Double-drugging via active and allosteric sites is a recently developed approach to overcome these obstacles. Herein, we provide the quantitative framework for double-drugging using two targets: Aurora A kinase (AurA) and Abl. Both kinases participate in various cellular pathways, and their dysregulation results in a multitude of cancers, such as breast cancer and leukemia. We find that both orthosteric and allosteric ligands exhibit preferred binding to the active or inactive states and that cooperativity occurs by shifting this active–inactive conformational equilibrium through long-range allosteric networks that are encoded for natural regulation of those kinases.

Intrigued by the synergistic effect of SKI and asciminib on Abl activity, we structurally characterized this ternary complex by cocrystallization, resulting in a 2.86 Å crystal structure of Abl64–510-SKI-asciminib [inactive, DFGin, BLBplus (29, 30)]. First, we note that the entire N-terminal lobe is ~30° twisted only for Abl64–510-SKI-asciminib, when aligned by the regulatory domains. Second, the α-C helix is adopting the “out” position resulting from this N-lobe twist, since an α-C helix “in position” would clash with strands β4 and β5. In consequence, the canonical salt bridge between K290 and E305, a hallmark of an active kinase, is broken in our structure, whereas D400 (DFG-motif) is positioned in the “in” position. We note, that the orthosteric site is fully occupied by SKI and the twisted N-lobe aids in forming this tightly packed binding pocket. In fact, K290 located on β3 strand is wrapping over SKI burying the inhibitor in Abl’s orthosteric site. Besides extensive van der Waals interactions between SKI and Abl, the quinazoline ring of SKI shares two hydrogen bonds with Abl, one between the side chain hydroxyl of T334 on β-strand 5 and N-2 of SKI as well as between the amide of M337 and N-0 of SKI. When compared to other closed Abl structures, we find an extended domain interface between SH3, linker, and N-lobe of the kinase domain, which explains the positive cooperativity between SKI and asciminib. Moreover, S248 (located on the linker) forms a hydrogen bond with D96 in the SH3 domain, which is only present in the ternary complex of Abl64–510-SKI-asciminib. We conclude that our complex of Abl64–510-SKI-asciminib represents the only example of a fully closed and inactive Abl structure.

>[2x]GNLFVALYDFVASGDNTLSITKGEKLRVLGYNHNGEWCEAQTKNGQGWVPSNYITPVNSLEKHSWYHGPVSRNAAEYLLSSGINGSFLVRESESSPGQRSISLRYEGRVYHYRINTASDGKLYVSSESRFNTLAELVHHHSTVADGLITTLHYPAPKRNKPTVYGVSPNYDKWEMERTDITMKHKLGGGQYGEVYEGVWKKYSLTVAVKTLKEDTMEVEEFLKEAAVMKEIKHPNLVQLLGVCTREPPFYIITEFMTYGNLLDYLRECNRQEVNAVVLLYMATQISSAMEYLEKKNFIHRDLAARNCLVGENHLVKVADFGLSRLMTGDTYTAHAGAKFPIKWTAPESLAYNKFSIKSDVWAFGVLLWEIATYGMSPYPGIDLSQVYELLEKDYRMERPEGCPEKVYELMRACWQWNPSDRPSFAEIHQAFETMFQESSISDEVEKEL> MTNESILESYSGVTPERKKSRMPAKLDWWQSATGLFLGLFMIGHMFFVSTILLGDNVMLWVTKKFELDFIFEGGKPIVVSFLAAFVFAVFIAHAFLAMRKFPINYRQYLTFKTHKDLMRHGDTTLWWIQAMTGFAMFFLGSVHLYIMMTQPQTIGPVSSSFRMVSEWMWPLYLVLLF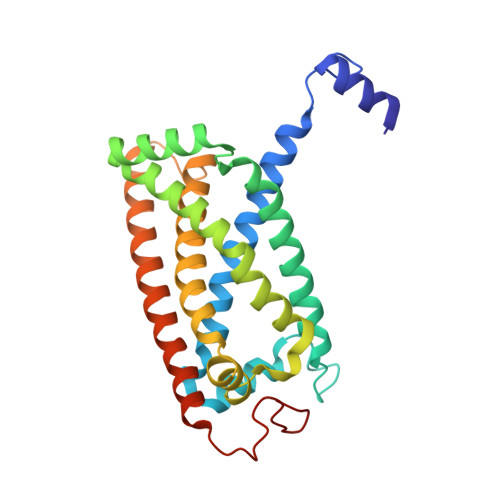AVELHGSVGLYRLAVKWGWFDGETPDKTRANLKKLKTLMSAFLIVLGLLTFGAYVKKGLEQTDPNIDYKYFDYKRTHHR> GSSHHHHHHSGDPASMIINNRNESQPRRVVVTGLGVVAPTGVGVNEFWNNIHNGKSGVSKYEWGRERFGFKSGAIGQVYGSDGNNKEFVLKSERKYLQFALDAAEMAMQDANLRPSDIDGRRFGVAIATAIADAAGMEECLLRITKGGKENI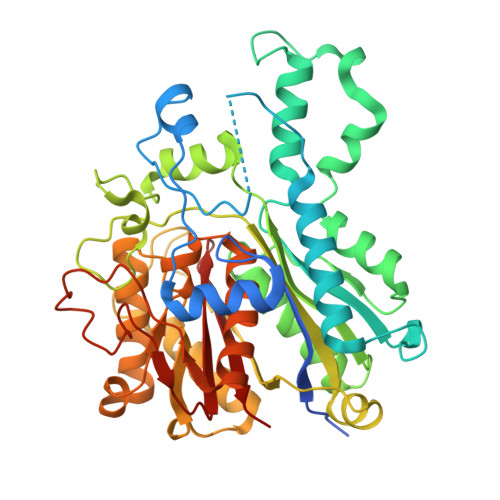HPDLIKSEDYDSFDFSSAATSVAKKYGASMSVSNISTGCAAGLDALGIAMEHIRYGRADIMLAGASEAPLCPLSIGSFEALGALSSRELENQQAATCPFSLERDGFVIAEGCGILILESYEHAKQRGAHIYAELAGYASVNNAYHMTDLPADGMAMARCIDMALKDAQISPSTVNYISAHGSSTAQNDINESNAIKFVLGESAFGIPINSLKSMTGHALAAANAIESVALCLEIEKQYVHPTINYQTPDPDCDLDYIPNQGCSYPIKTALKLSSGFSGIHSVIVMRAVDNA> MSLGRKQQYGTLASIAAKLGISRTTVSNAYNRPEQLSAELRQRILDTAEDMGYLGPDPVARSLRTRRAGAIGVLLTEDLTYAFEDMASVDFLAGV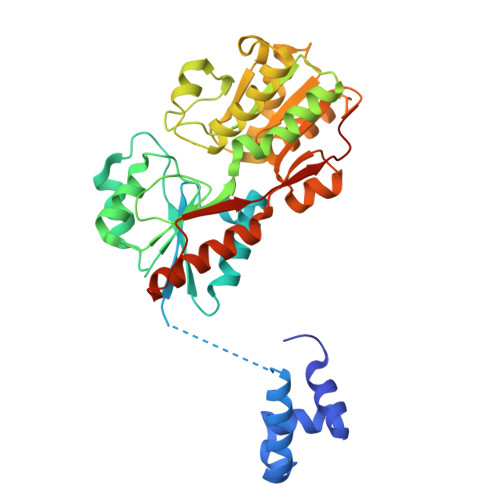AQAAGDTQLTLIPASPASSVDHVSAQQLVNNAAVDGVVIYSVAKGDPHIDAIRARGLPAVIADQPAREEGMPFIAPNNRKAIAPAAQALIDAGHRKIGILSIRLDRANNDGEVTRERLENAQYQVQRDRVRGAMEVFIEAGIDPGTVPIMECWINNRQHNFEVAKELLETHPDLTAVLCTVDALAFGVLEYLKSVGKSAPADLSLTGFDGTHMALARDLTTVIQPNKLKGFKAGETLLKMIDKEYVEPEVELETSFHPGSTVAEGHHHHHH> GMTDNHIDVLINGCGIGGAMLAYLLGRQGHRVVVVEQARRERAINGADLLKPAGIRVVEAAGLLAEVTRRGGRVRHELEVYHDGELLRYFNYSSVDARGYFILMPCESLRRLVLEKIDGEATVEMLFETRIEAVQRDERHAIDQVRLNDGRVLRPRVVVGADGIASYVRRRLLDIDVERRPYPSPMLVGTFALAPCVAERNRLYVDSQGGLAYFYPIGFDRARLVVSFPREEARELMADTRGESLRRRLQRFVGDESAEAIAAVTGTSRFKGIPIGYLNLDRYWADNVAMLGDAIHNVHPITGQGMNLAIEDASALADALDLALRDACALEDALAGYQAERFPVNQAIVSYGHALATSLEDRQRFAGVFDTALQGSSRTPEALGGERSYQP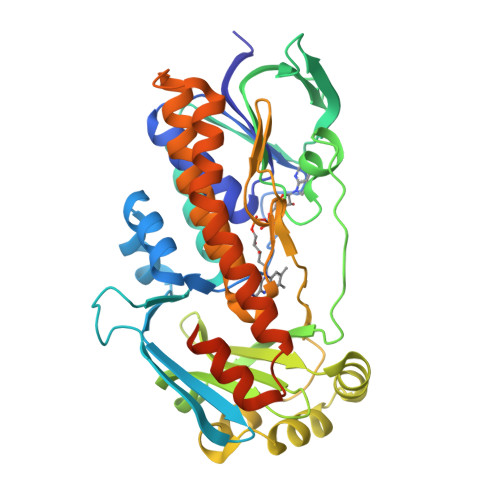VRSPAPLG>MKMLEQLEKKLGYTFKDKSL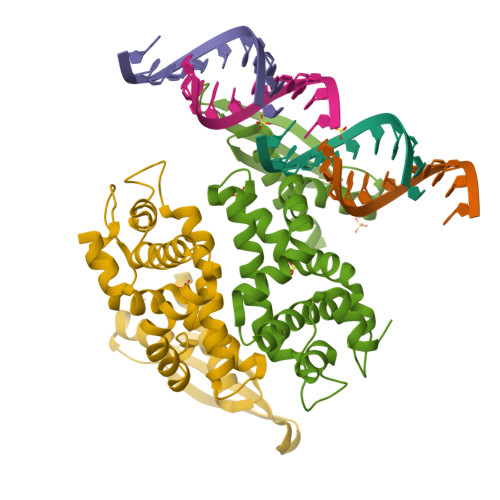LEKALTHVSYSKKEHYETLEFLGDALVNFFIVDLLVQYSPNKREGFLSPLKAYLISEEFFNLLAQKLELHKFIRIKRGKINETIIGDVFQALWAAVYIDSGRDANFTRELFYKLFKEDILSAIKEGRVKKDYKTILQEITQKRWKERPEYRLISVEGPHHKKKFIVEAKIKEYRTLGEGKSKKEAEQRAAEELIKLLEESE[2x]>[4x]MLGNDTVEIKDGRFFIDGYDAIELAEKFGTPLYVMSEEQIKINYNRYIEAFKRWEEETGKEFIVAYAYKANANLAITRLLAKLGCGADVVSGGELYIAKLSNVPSKKIVFNGNCKTKEEIIMGIEANIRAFNVDSISELILINETAKELGETANVAFRINPNVNPKTHPKISTGLKKNKFGLDVESGIAMKAIKMALE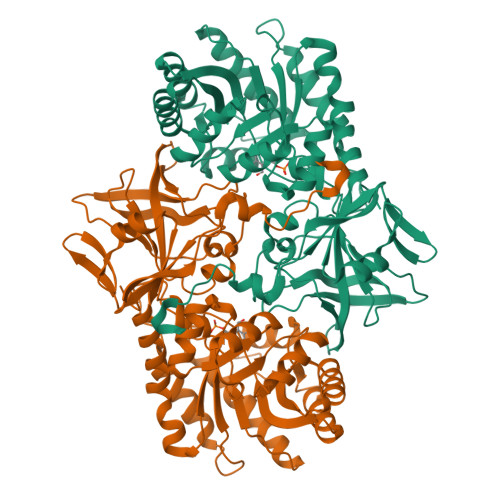MEYVNVVGVHCHIGSQLTDISPFIEETRKVMDFVVELKEEGIEIEDVNLGGGLGIPYYKDKQIPTQKDLADAIINTMLKYKDKVEMPNLILEPGRSLVATAGYLLGKVHHIKETPVTKWVMIDAGMNDMMRPAMYEAYHHIINCKVKNEKEVVSIAGGLCESSDVFGRDRELDKVEVGDVLAIFDVGAYGISMANNYNARGRPRMVLTSKKGVFLIRERETYADLIAKDIVPPHLL> MEEHTEAGSAPEMGAQKALIDNPADILVIAAYFLLVIGVGLWSMCRTNRGTVGGYFLAGRSMVWWPVGASLFASNIGSGHFVGLAGTGAASGLAVAGFEWNALFVVLLLGWLFAPVYLTAGVITMPQYLRKRFGGRRIRLYLSVLSLFLYIFTKISVDMFSGAVFIQQALGWNIYASVIALLGITMIYTVTGGLAALMYTDTVQTFVILGGACILMGYAFHEVGGYSGLFDKYLGAATSLTVSEDPAVGNISSFCYRPRPDSYHLLRHPVTGDLPWPALLLGLTIVSGWYWCSDQVIVQRCLAGKSLTHIKAGCILCGYLKLTPMFLMVMPGMISRILYPDEVACVVPEVCRRVCGTEVGCSNIAYPRLVVKLMPNGLRGLMLAVMLAALMSSLASIFNSSSTLFTMDIYTRLRPRAGDRELLLVGRLWVVFIVVVSVAWLPVVQAAQGGQLFDYIQAVSSYLAPPVSAVFVLALFVPRVNEQGAFWGLIGGLLMGLARLIPEFSFGSGSCVQPSACPAFLCGVHYLYFAIVLFFCSGLLTLTVSLCTAPIPRKHLHRLVFSLRHSKEEREDLDADEQQGSSLPVQNGCPESAMEMNEPQAPAPSLFRQCLLWFCGMSRGGVGSPPPLTQEEAAAAARRLEDISEDPSWARVVNLNALLMMAVAVFLWGFYA;> MSALSLLILGLLTAVPPASCQQGLGNLQPWMQGLIAVAVFLVLVAIAFAVNHFWCQEEPEPAHMILTVGNKADGVLVGTDGRYSSMAASFRSSEHENAYENVPEEEGKVRSTPM

The uptake of glucose against its concentration gradient is mediated by the sodium-dependent glucose cotransporters (SGLT). These transporters utilize the electrochemical gradient to drive the uphill transport of glucose and play essential roles in human health. SGLT1 (SLC5A1) and SGLT2 (SLC5A2) are two important subtypes of this family, and their physiological functions are well-documented. Pioneering structural work on the bacterial homolog vSGLT from Vibrio parahaemolyticus revealed that SGLT proteins have 14 transmembrane helices, which assemble into a LeuT-like fold.

To visualize the substrate-bound structure of hSGLT2, we supplemented methyl alpha-d-galactopyranoside (AMG) into the hSGLT2GFP-MAP17nb protein in nanodisc. Subsequent single particle analysis generated reconstruction of the hSGLT2-AMG complex at 3.33 Å resolution. We observed that AMG is bound in an occluded substrate-binding site and we modeled the AMG into the density according to the structures of the vSGLT-galactose complex8 and the hSGLT2-empagliflozin complex10. The structure and conformation of the hSGLT2-AMG complex are overall similar to those of the hSGLT1-4D4FDG complex. We did not observe densities for sodium ions in these structures, likely due to their low resolutions. MAP17 is an essential subunit for the glucose uptake activity of hSGLT2 but not hSGLT115. Because MAP17 interacts with TM13 of hSGLT2, which is part of the less-mobile region that shows little conformational changes between different states of the hSGLT2-MAP17 complex, the conformation of MAP17-TM13 also stays the same. In agreement with this, we found similar structural changes of the Na2 and Na3 sites in hSGLT2, even though the Na3 site of hSGLT2 is not functional, indicating the Na3 site likely enhances the sodium and sugar affinity thermodynamically.>[3x]GAMGSKLSYTSFVQMVEDERS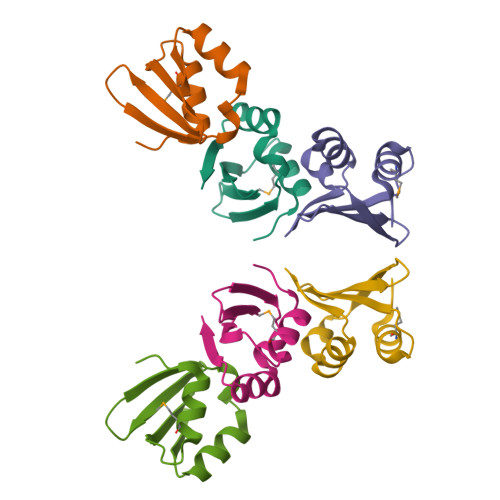VVSEVVIRDDGVLRVYTKDGRVYEVDAPWAVNDSQLIEKLVSKGIKVSGER> TIIFGF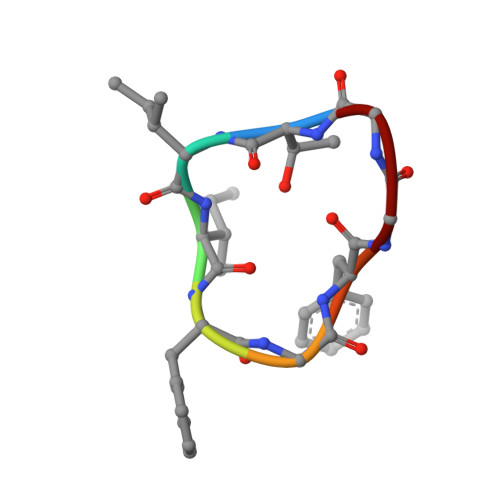GG>MSPTGNYLNAITNRRTIYNLKPELPQGVGLDDVKRTVHVILKNTPTAFNSQVNRAVIIVGDTHKRIWDAVASAMPTAEAKKRPESCRDEAYGSVIFFTDLGPTEKLQRDFPALAAAFPTCAAHTTGAVQIQSWTALELLGLGANLQHYNDYVKSALPQDVPIA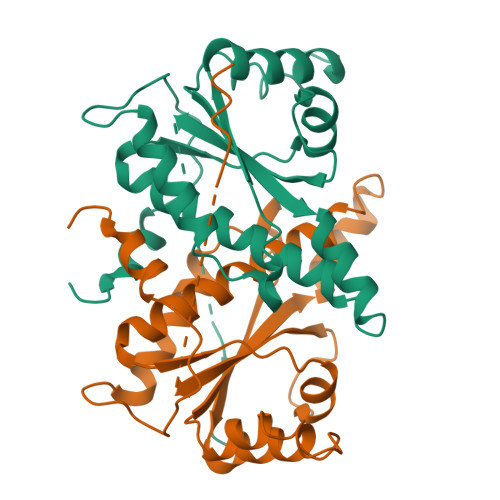WTVQSQLVFGVPTALPEEKTFINNVINVYH[2x]>MLVSVYLALLVACVGQAHSQANLMRLKSDLFNRSPMYPGPTKDDPLTVTLGFTLQDIVKVDSSTNEVDLVYYEQQRWKLNSLMWDPNEYGNITDFRTSAADIWTPDITAYSSTRPVQVLSPQIAVVTHDGSVMFIPAQ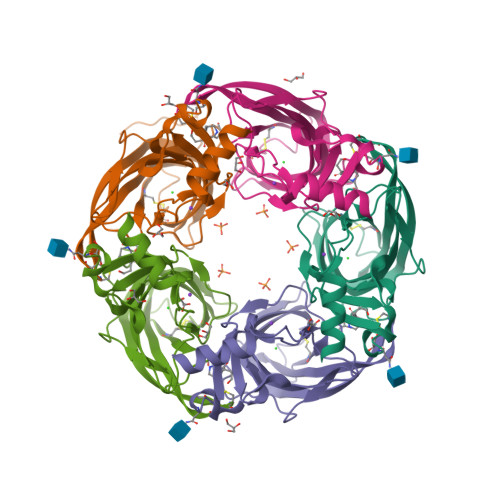RLSFMCDPTGVDSEEGVTCAVKFGSWVYSGFEIDLKTDTDQVDLSSYYASSKYEILSATQTRQVQHYSCCPEPYIDVNLVVKFRERRAGNGFFRNLFDENLYFQGHHHHHH[10x]>MAQSVTADPSPPITDTNKLNKYSSRITEPKSQGGSQAILHGVGLSDDDLLKPQIGISSVWYEGNTCNMHLLKLSEAVKEGVENAGMVGFRFNTIGVSDAISMGTRGMCFSLQSRDLIADSIETVMSAQWYDGNISIPGCDKNMPGTIMAMGRLNRPGIMVYGGTIKPGHFQDKTYDIVSAFQSYGEFVSGSISDEQRKTVLHHSCPGAGACGGMYTANTMASAIEAMGMSLPYSSSIPAEDPLKLDECRLAGKYLLELLKMDLKPRDIITPKSLRNAMVSVMALGGSTNAVLHLIAIARSVGLELTLDDFQKVSDAVPFLADLKPSGKYVMEDIHKIGGTPAVLRYLLELGLMDGDCMTVTGQTLAQNLENVPSLTEGQEIIRPLSNPIKETGHIQILRGDLAPDGSVAKITGKEGLYFSGPALVFEGEESMLAAISADPMSFKGTVVVIRGEGPKGGPGMPEMLTPTSAIMGAGLGKECALLTDGRFSGGSHGFVFGHICPEAQEGGPIGLIKNGDIITIDIGAARIDTQVSPEEMNDRRKKWTAPAYKVNRGVLYKYIKNVQSASDGCVTDE[2x]

Dihydroxy acid dehydratase (DHAD) is the third enzyme in the plant branched-chain amino acid biosynthetic pathway and the target for commercial herbicide development. We have previously reported the discovery of fungal natural product aspterric acid (AA) as a submicromolar inhibitor of DHAD through self-resistance gene directed genome mining. Here, we reveal the mechanism of AA inhibition on DHAD and the self-resistance mechanism of AstD, which is encoded by the self-resistance gene astD. Our structural and kinetic analysis of the mutant AthDHADs has validated the hypothesis that larger hydrophobic amino acids surrounding the active-site entrance enhance resistance to AA.

To determine if small-to-large amino acid mutations at these hydrophobic residues can decrease active site volume and increase resistance to AA, we generated multiple mutations at V496, V497, and I177 in AthDHAD followed by kinetic and structural characterizations. The substitutions of V496L and V497I may push the loop where G490 is located toward the center of the channel. Additionally, the inhibitory concentration (IC50) of AA for the V497L, V497I, and V497F mutants were determined as 0.059, 0.0733, and 1.25 μM, respectively. To probe the acquired resistance mechanism of AthDHAD mutants, we determined the crystal of AthDHAD–I177F (2.45 Å), AthDHAD–V178W (1.77 Å), AthDHAD–V496W (1.59 Å), and AthDHAD–V497F (1.87 Å). In the crystal structures of I177F, V178W, V496W, and V497F, the occupancy of [2Fe–2S] cluster is 0.64, 0.72, 0.63, and 0.77, respectively. The overall structures of the AthDHAD mutants I177F, V178W, V496W, and V497F displayed high similarity with the wild-type AthDHAD, with the RMSD of 0.123 Å (888 core Cα atoms), 0.275 Å (994 core Cα atoms), 0.142 Å (1,034 core Cα atoms), and 0.283 Å (994 core Cα atoms), respectively. The obvious difference was in loop 490–497, which forms the side wall at the narrowest point of the substrate channel. In the V497F structure, the benzene ring of F497 induces F495 to rotate about 53° which change the shape of loop 489–493 and make it close to the V178 at the channel entrance. As a result, this mutant also affects the accession of AA to the active site.>[2x]SNADLLVPKLTASVTDGAVGVTVDAPVS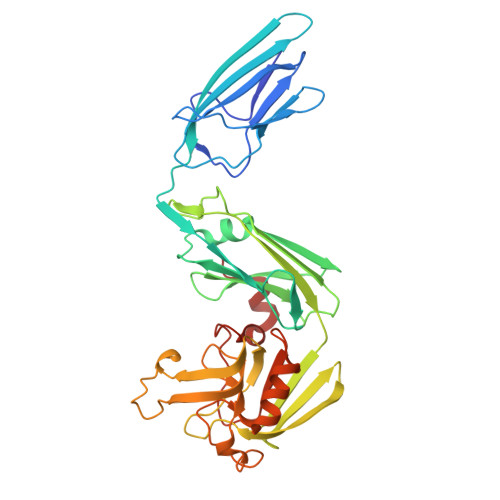VTAADGVLAAVTMVNDNGRPVAGRLSPDGLRWSTTEQLGYNRRYTLNATALGLGGAATRQLTFQTSSPAHLTMPYVMPGDGEVVGVGEPVAIRFDENIADRGAAEKAIKITTNPPVEGAFYWLNNREVRWRPEHFWKPGTAVDVAVNTYGVDLGEGMFGEDNVQTHFTIGDEVIATADDNTKILTVRVNGEVVKSMPTSMGKDSTPTANGIYIVGSRYKHIIMDSSTYGVPVNSPNGYRTDVDWATQISYSGVFVHSAPWSVGAQGHTNTSHGCLNVSPSNAQWFYDHVKRGDIVEVVNTVGGTLPGIDGLGDWNIPWDQWRAGNAKA>MIVRSFIYEPFQIPSGSMMPTLLIGDFILVEKFAYGIKDPIYQKTLIETGHPKRGDIVVFKYPEDPKLDYIKRAVGLPGDKVTYDPVSKELTIQPGCSSGQACENALPVTYSNVEPSDFVQTFSRRNGGEATSGFFEVPKNETKENGIRLSERKETLGDVTHRILTVPIAQDQVGMYYQQPGQQLATWIVPPGQYFMMGDNRDNSADSRYWGFVPEANLVGRATAIWMSFDKQEGEWPTGLRLSRIGGIH[2x]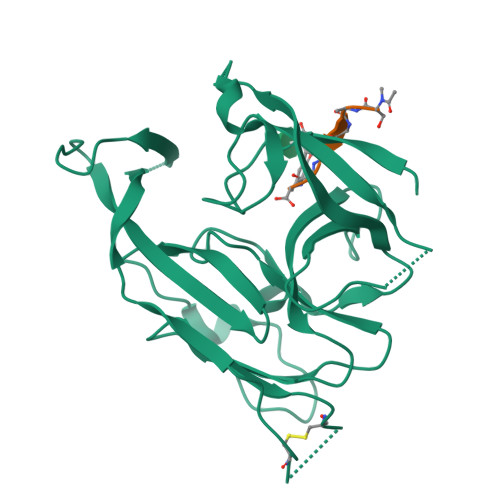;>SAGXAY[2x]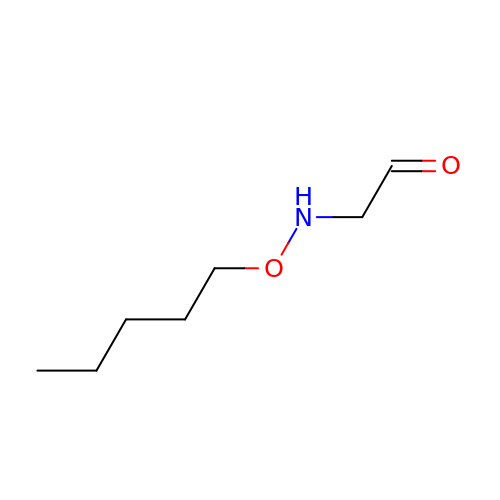PENTYLOXYAMINO-ACETALDEHYDE | C7 H15 N O2 | PKNNPRVGISCRDL-UHFFFAOYSA-N N-[5-(3-{2-[(cyclopropylmethyl)amino]pyrimidin-4-yl}-7-[(dimethylamino)methyl]-6-methylimidazo[1,2-a]pyridin-2-yl)-2-fluorophenyl]methanesulfonamide 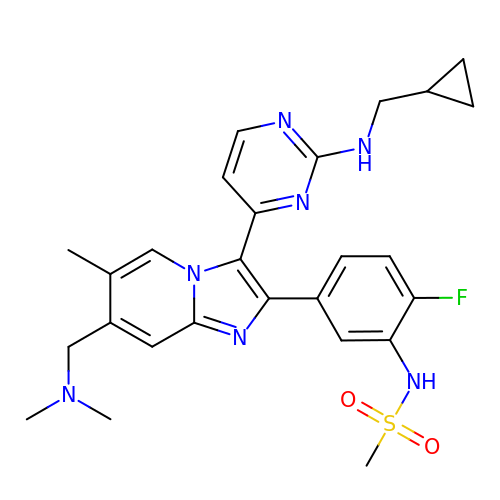| C26 H30 F N7 O2 S | LDISLUXUWYPJIZ-UHFFFAOYSA-N> EVTIEAVPPQ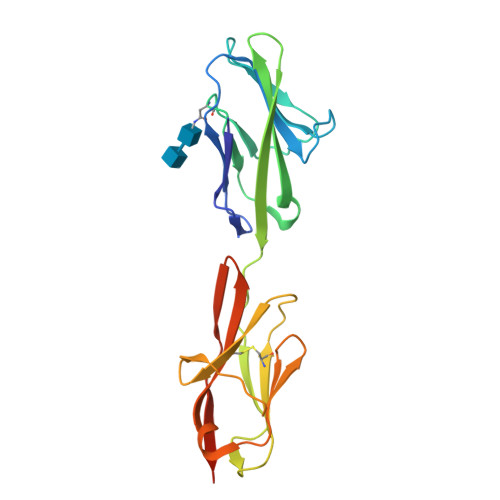VAEDNNVLLLVHNLPLALGAFAWYKGNPVSTNAEIVHFVTGTNKTTTGPAHSGRETVYSNGSLLIQRVTVKDTGVYTIEMTDENFRRTEATVQFHVHQPVTQPSLQVTNTTVKELDSVTLTCLSNDIGANIQWLFNSQSLQLTERMTLSQNNSILRIDPIKREDAGEYQCEISNPVSVKRSNSIKLDIIFDPHHHHHH> EAASSSDADGKEVGSSGEGNRATGGKWRRPSLAQQRARRAQLPPAFDVVHWNDEDISRGHLLRVLHRDTFVVLDYHRQARMLTEEGNKAERVVSVMLPAVYTARFLAVLEGRSEKVEVHSRYTNATFTPNPAAPYTFTLKCTSTRPAQQKQQVA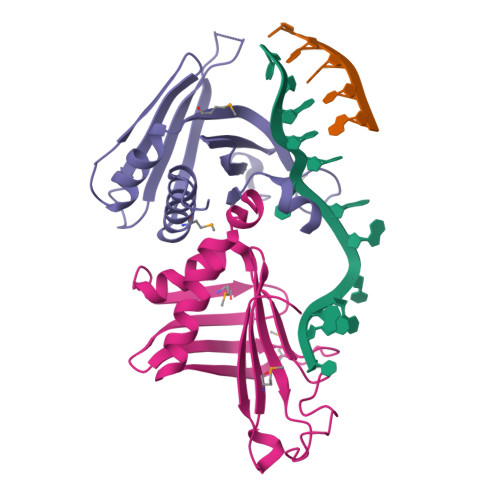GEEGDETFEWTVEFDVAESLMLQRFLTQALHYNTGFARTSV;> ASTFSGVQSLPKFEIHDVRDDPAEGTMTRVAVDGKLLLISQYPQLGPRKVDPNDLSPQFDADRRISVRLRHVDLAYLVGVCKERVPRHRMETKAYTLDFEKSAQGYHLHGKVHRVASQRMEDWSVKFDNHFAVTLEHFLESALDESFGFRQHYATRAAEGGEKIAATSSAEGGARRKRSVSDTSRYH>[3x]EVNEKAPAQARPTVFRWTGGGKEVYLSGSFNNWSKLPLTRSQNNFVAILDL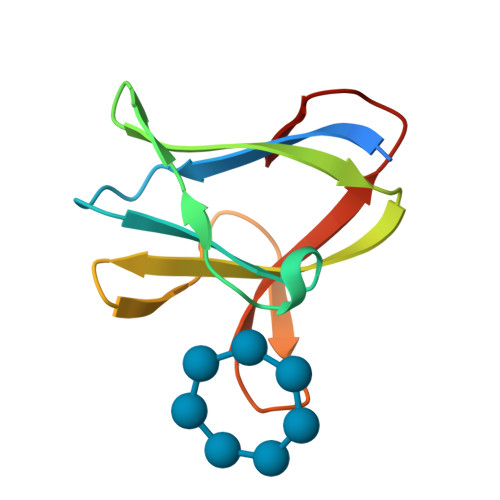PEGEHQYKFFVDGQWTHDPSEPIVTSQLGTVNNIIQVKKTDFEVF>[2x]MAHHHHHHMRGRS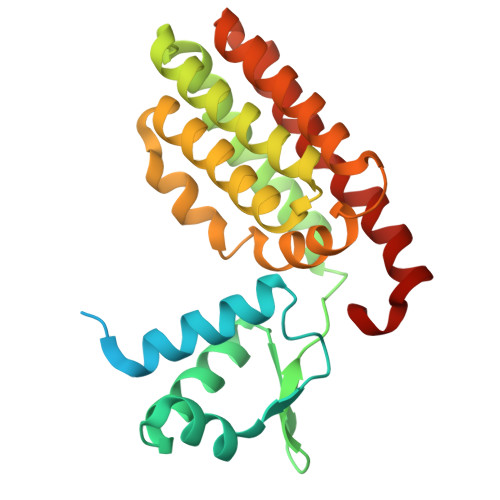AQPALEKQKNVADTESGAATGVKARTLPSRVAGVQRVTTAKLIYHELQQQIIRMELLPGTPLNEKALTEKYGVSRTPVREALIRLAEDRLVDVFPQSGTFVARIPVDAIPEAVVIRQALEGETAERAAANSTAAAIEKLDELIHLQTFYARKDKPGPFHETDDAFHETIAEIAGYPGIWQHLKPVKMQIDRARRMTMPILGRMEQVLREHHAIRDAISARDVHAAREAMKHHLSAVLPDIDELRKSRPDYFA CYCLOPENTYL N-[(2S)-1-[(2S,4R)-2-[[(4R)-8-HYDROXY-1,6,10-TRIOXA-5$L^{4}-BORASPIRO[4.5]DECAN-4-YL]CARBAMOYL]-4-ISOQUINOLIN-1-YLOXY-PYRROLIDIN-1-YL]-3,3-DIMETHYL-1-OXO-BUTAN-2-YL]CARBAMATE | C32 H44 B N4 O9 | 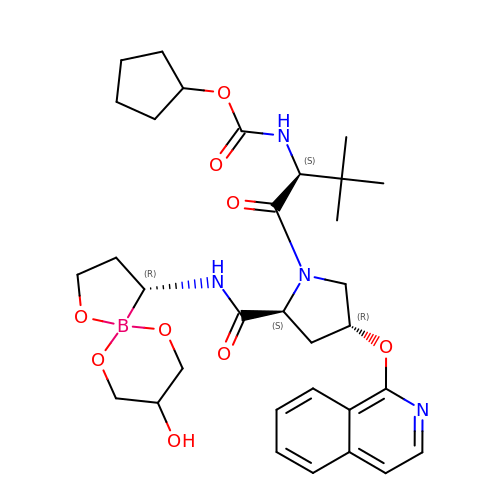MSXWUFQOFQGEEP-GYUKIKGESA-N>MSDFLPGLEGVPATKSAISFIDGEKGILSYRGYPLETLAENSTFEETTLLLLDGELPTKKALNDFSQQLKDNYRIKYHIRQMMRHFPHTGHPMDMLQTAVSSLGMFYPGTECLTDANSCEDLDYVRNMTVNIIAQMAPLVAMWEHIRNGWDPVNPKHDLSVAENLLYMFNGEEPDPLMAKIMDVCLILHAEHTLNASTFAALVAGSTLATPYSVISAAIGTLSGPLHGGANQRVVGMLQEIGSPKNVESWVDEKLKNKEVIWGMGHREYKVKDPRATILHKLVEQLVAERGGHLDDMFD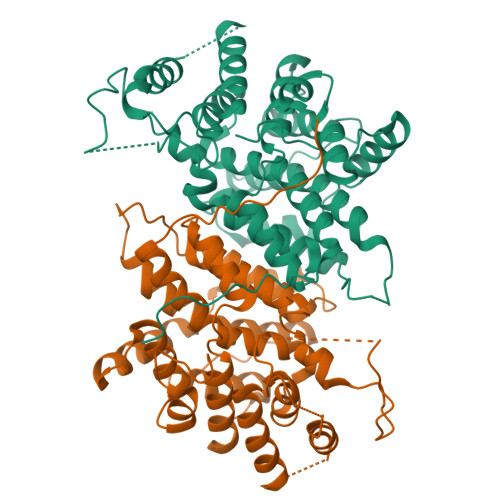TALKLEEVCADRLGHKGVYPNVDFYSGILYSEMGIPEDEFTALFAVARSAGWLAHWREQISDNRIYRPTQIYVGSDMRDYTPIEERLVPRLEHHHHHH[12x]~{N}-[(1~{R})-4-[4-[(6-fluoranyl-1,3-benzothiazol-5-yl)amino]thieno[2,3-d]pyrimidin-6-yl]cyclohex-3-en-1-yl]cyclopropanecarboxamide 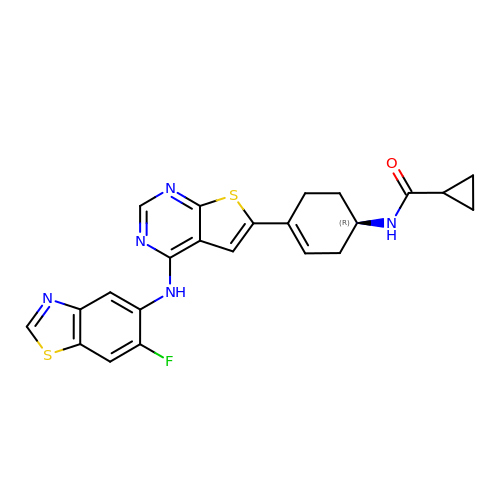| C23 H20 F N5 O S2 | HBUARMMKBQMRBE-AWEZNQCLSA-N>[4x]MGSTGNAEIQIIPTHSSDEEANLFAMQLASAAVLPMALKAAIELDVLEIMAKSVPPSGYISPAEIAAQLPTTNPEAPVMLDRVLRLLASYSVVTYTLRELPSGKVERLYGLAP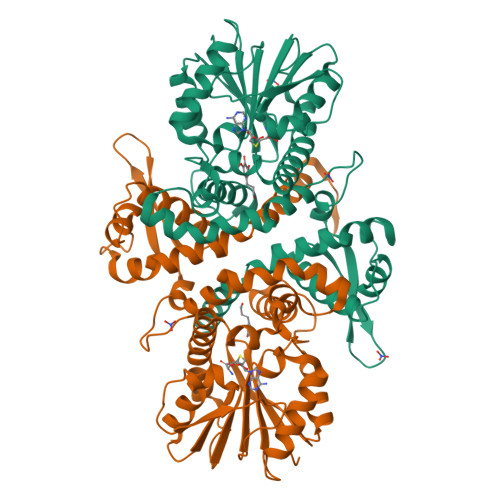VCKFLTKNEDGVSLAPFLLLATDKVLLEPWFYLKDAILEGGIPFNKAYGMNIWDYFGTDHRINKVFNKGMSSNSTITMKKILEMYNGFEGLTTIVDVGGGTGAVASMIVAKYPSINAINFDLPHVIQDAPAFSGVEHLGGDMFDGVPKGDAIFIKWICHDWSDEHCLKLLKNCYAALPDHGKVIVAEYILPPSPDPSIATKVVIHTDALMLAYNPGGKERTEKEFQALAMASGFRGFKVASCAFNTYVMEFLKTA> MDGSGEQPRGGGPTSSEQIMKTGALLLQGFIQDRAGRMGGEAPELAL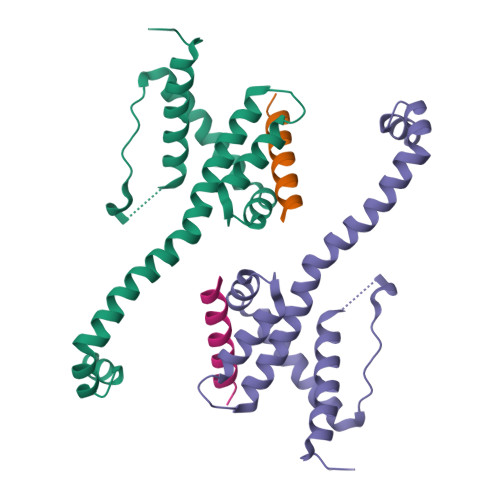DPVPQDASTKKLSESLKRIGDELDSNMELQRMIAAVDTDSPREVFFRVAADMFSDGNFNWGRVVALFYFASKLVLKALSTKVPELIRTIMGWTLDFLRERLLGWIQDQGGWDGLLSYFGSS;> XQEDIIRNIARHLAQVGDSMD Sterile alpha motif and HD domain-containing protein 1 (SAMHD1) is an important regulator of cellular 2′-deoxynucleoside-5′-triphosphate (dNTP) in mammalian cells. Although the HD-domain contains the active site, dNTP hydrolysis requires assembly of SAMHD1 into homo-tetramers. Here, sequences at the N and C termini of the HD-domain stabilise inter-monomer protein–protein interactions and incorporate four pairs of allosteric nucleotide-binding sites, AL1 and AL2, which regulate the enzyme through combined binding of G-based (AL1) and 2′-deoxynucleoside (AL2) triphosphates. Using combined biophysical and X-ray structural studies incorporating nucleotide analogues along with mutagenesis experiments we have now discovered that SAMHD1 uses a bi-metallic Fe–Mg centre to catalyse dNTP hydrolysis in a reaction similar to those catalysed by HD domains in both human and bacterial phosphodiesterase PDE enzymes.

Therefore, given our observations, we sought to validate our findings and confirm the position of metal ions by substitution of Mg2+ with Mn2+ and identify ion positions using diffraction methods. Although Mg2+ is essential for SAMHD1 catalysis, Mn2+ still supports dNTP hydrolysis with similar catalytic parameters, as is observed in other phosphohydrolase enzymes. Therefore, Mg2+ ions were substituted with Mn2+ ions in the SAMHD1–dNMPNPP co-crystallisation conditions and the structure of D137N-SAMHD1(109-626)-Mn-XTP-dAMPNPP complex was determined at 2.25 Å. 2Fo − Fc maps contoured at high σ were then used to locate and confirm the position of the highly X-ray scattering Mn2+ ions in the active and allosteric sites in the structure. Co-crystal structures were determined using either wild-type (wt) wt-SAMHD1(109-626) or a D137N-SAMHD1(109-626) AL1 allosteric site mutant that generally produced higher resolution diffraction than wt co-crystals. A further effect of the D137N substitution is that D137N-SAMHD1 is activated by xanthosine-5′-triphosphate (XTP) rather than GTP through AL1-binding but nevertheless maintains comparable catalytic parameters for dNTP hydrolysis as those observed for wt-SAMHD1 and GTP.

>GSQIHVDTMKVINDPIHGHIELHPLLVRIINTPQFQRLRYIKQLGGGYYVFPGASHNRFEHSLGVGYLAGCLVHALGEKQPELQISERDVLCVQIAGLCHDLGHGPFSHMFDGRFIPLARPEVKWTHEQGSVMMFEHLINSNGIKPVMEQYGLIPEEDICFIKEQIVGPLESPVEDSLWPYKGRPENKSFLYEIVSNKRNGIDVDKWDYFARDCHHLGIQNNFDYKRFIKFARVCEVDNELRICARDKEVGNLYDMFHTRNSLHRRAYQHKVGNIIDTMITDAFLKADDYIEITGAGGKKYRISTAIDDMEAYTKLTDNIFLEILYSTDPKLKDAREILKQIEYRNLFKYVGETQPTGQIKIKREDYESLPKEVASAKPKVLLDVKLKAEDFIVDVINMDYGMQEKNPIDHVSFYCKTAPNRAIRITKNQVSQLLPEKFAEQLIRVYCKKVDRKSLYAARQYFVQWCADRNFTKPQDGDVIAPLITPQKKEWNDSTSVQNPTRLREASKSRVQLFKDDPM[2x]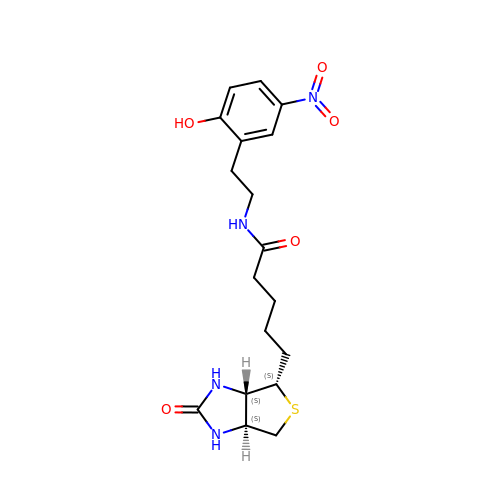N-[2-(2-hydroxy-5-nitrophenyl)ethyl]-5-[(3aS,4S,6aS)-2-oxohexahydro-1H-thieno[3,4-d]imidazol-4-yl]pentanamide | C18 H24 N4 O5 S | GGNOUTGIVZKNRF-KMFMINBZSA-N> MSSDSFQRQLVQRTNTLNSSIDNA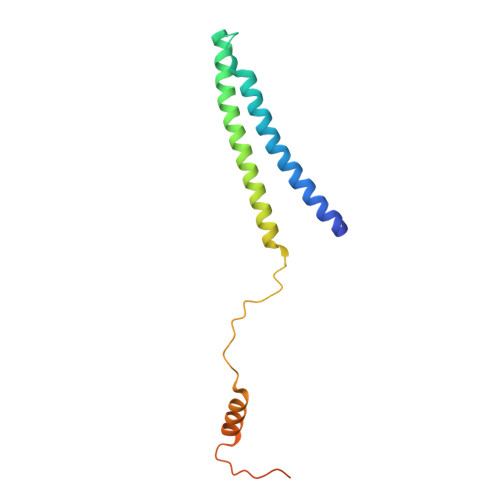TLTILSRFQDILDIAINEGKDKYTVAPEVYQIECHTVSMVRAVEQLLDVSRQIKSYWLTNSLSTSFPTVDYSEPDLEKVKRTLTKLQNHLLEVSLIEPEASETTEAPTVSDT> MAIQSKYSNTQVESLIAEILVVLEKHKAPTD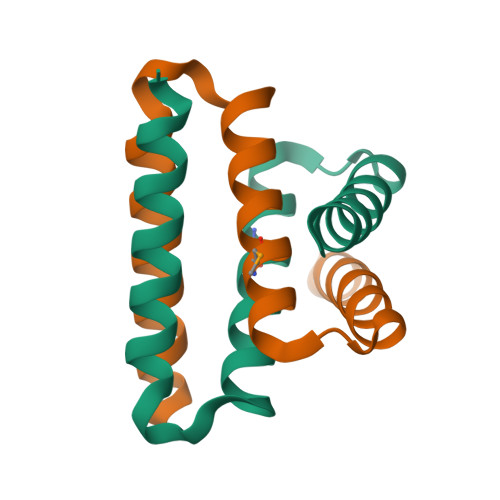LSLMALGNCVTHLLERKVPSESRQAVAEQFAKALAQSVKSNLEHHHHHH1-[1-(3,5-dimethoxyphenyl)indolizin-3-yl]ethanone | C18 H17 N O3 | 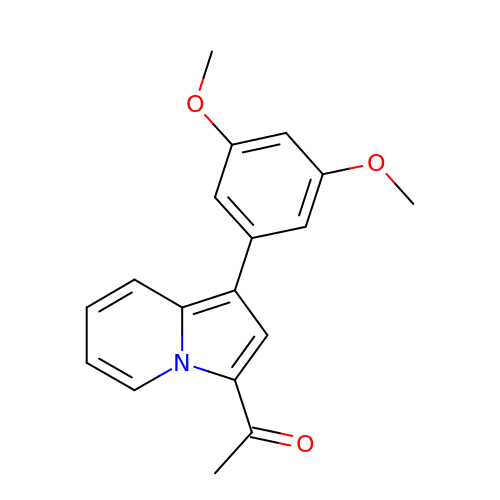FTNILURDQGAJNO-UHFFFAOYSA-N> GPLGSELSRQIKAAASTLEDIEVKDDEWAVDMSEEAIRARAKELEVNSELTQLDEYGEWILEQAGEDKENLPSDVELYKKAAELDVLNDPKIGCVLAQCLFDEDIVNEIAEHNAFFTKILVTPEYEKNFMGGIERFL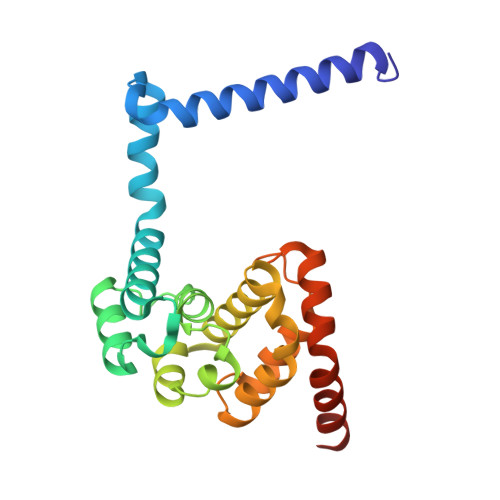GLEHKDLIPLLPKILVQLYNNDIISEEEIMRFGTKSSKKFVPKEVSKKVRRAAKPFITWLETAESDDDEEDDE The periplasmic binding protein (PBP) CeuE1 is an important component of the Fe(III) uptake system in Campylobacter jejuni, a commensal Gram-negative bacterium in the avian gut, but a common source of food poisoning in humans. CeuE, an integral part of the CeuBCDE ABC transporter of C. jejuni, is responsible for capturing Fe(III)-siderophore complexes in the periplasm for delivery to their respective inner membrane transporter. C. jejuni does not itself synthesize siderophores, but capitalizes on their secretion by other bacteria, such as E. coli. Here we report a combined solution and structural study of a series of synthetic tetradentate analogues of the enterobactin-derived bis(2, 3-dihydroxybenzoyl-L-Ser), to explore the ligand-binding promiscuity of CeuE, both wild type and with mutations of the Fe(III) binding residues H227 and Y288.

Fe(III) complexes of 5-LICAM4−, 6-LICAM4− and 8-LICAM4− were co-crystallized with CeuE and their crystal structures determined. The linkers between the two catecholate binding units are well ordered, with B-values close to the average value for each structure, in spite of the linker pointing toward the solvent with essentially no contacts to the protein. The longer linker of 8-Lic is notably well ordered considering its length and inherent potential for flexibility. This tolerance of longer linkers can be rationalized by the lack of protein contacts observed for the linker region in the structures. The structural differences can be quantified by calculating the mean planes defined by the six carbon atoms of the two catecholate rings, and measuring their inter-planar angle which is 97°, 111°, 110° and 110° in CFe-4-Lic, CFe-5-Lic, CFe-6-Lic and CFe-8-Lic, respectively. In contrast, the longer and more flexible linkers in Fe-5-Lic, Fe-6-Lic and Fe-8-Lic can adapt to both the geometric requirements of the Fe(III) center and the binding pocket of CeuE. Since the inter-planar angle between the catecholamide units in the CFe-6-Lic and CFe-8-Lic structures is identical (110°), the higher Kd value obtained for Fe-8-Lic is likely to reflect the higher entropic cost upon binding due to the greater number of conformational degrees of freedom in its linker. In addition, the affinities of CeuE for Fe-4-Lic, Fe-5-Lic, Fe-6-Lic and Fe-8-Lic were determined using fluorescence quenching, which yielded dissociation constants of 21 ± 6 nM, < 10 nM, 33 ± 8 nM and 58 ± 8 nM, respectively.

> PAMLPISMSDEGDSFLVKDSLGENKIPKNPSKVVILDLGILDTFDALKLNDKVVGVPAKNLPKYLQQFKNKPSVGGVQQVDFEAINALKPDLIIISGRQSKFYDKLKEIAPTLFVGLDNANFLSSFENNVLSVAKLYGLEKEALEKISDIKNEIEKAKSIVDEDKKALIILTNSNKISAFGPQSRFGIIHDVLGINAVDENIKVGTHGKSINSEFILEKNPDYIFVVDRNVILGNKERAQGILDNALVAKTKAAQNKKIIYLDPEYWYLASGNGLESLKTMILEIKNAVK>MADYKDDDDKSGRMLNNLTDCEDGDGGANPGDGNPKESSPFINSTDTEKGKEYDGKNMALFEEEMDTSPMVSSLLSGLANYTNLPQGSREHEEAENNEGGKKKPVQAPRMGTFMGVYLPCLQNIFGVILFLRLTWVVGIAGIMESFCMVFICCSCTMLTAISMSAIATNGVVPAGGSYYMISRSLGPEFGGAVGLCFYLGTTFAGAMYILGTIEILLAYLFPAMAIFKAEDASGEAAAMLNNMRVYGTCVLTCMATVVFVGVKYVNKFALVFLGCVILSILAIYAGVIKSAFDPPNFPICLLGNRTLSRHGFDVCAKLAWEGNETVTTRLWGLFCSSRFLNATCDEYFTRNNVTEIQGIPGAASGLIKENLWSSYLTKGVIVERSGMTSVGLADGTPIDMDHPYVFSDMTSYFTLLVGIYFPSVTGIMAGSNRSGDLRDAQKSIPTGTILAIATTSAVYISSVVLFGACIEGVVLRDKFGEAVNGNLVVGTLAWPSPWVIVIGSFFSTCGAGLQSLTGAPRLLQAISRDGIVPFLQVFGHGKANGEPTWALLLTACICEIGILIASLDEVAPILSMFFLMCYMFVNLACAVQTLLRTPNWRPRFRYYHWTLS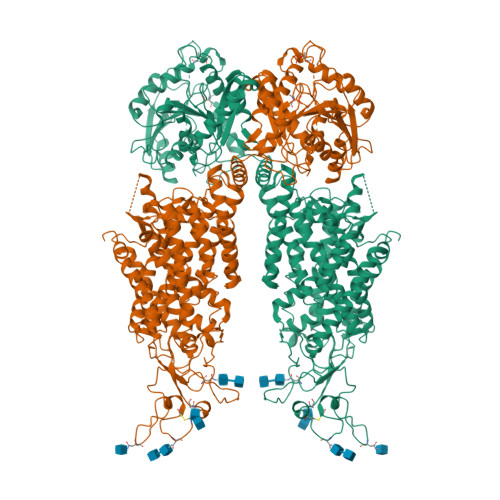FLGMSLCLALMFICSWYYALVAMLIAGLIYKYIEYRGAEKEWGDGIRGLSLSAARYALLRLEEGPPHTKNWRPQLLVLVRVDQDQNVVHPQLLSLTSQLKAGKGLTIVGSVLEGTFLENHPQAQRAEESIRRLMEAEKVKGFCQVVISSNLRDGVSHLIQSGGLGGLQHNTVLVGWPRNWRQKEDHQTWRNFIELVRETTAGHLALLVTKNVSMFPGNPERFSEGSIDVWWIVHDGGMLMLLPFLLRHHKVWRKCKMRIFTVAQMDDNSIQMKKDLTTFLYHLRITAEVEVVEMHESDISAYTYEKTLVMEQRSQILKQMHLTKNEREREIQSITDESRGSIRRKNPANTRLRLNVPEETAGDSEEKPEEEVQLIHDQSAPSCPSSSPSPGEEPEGEGETDPEKVHLTWTKDKSVAEKNKGPSPVSSEGIKDFFSMKPEWENLNQSNVRRMHTAVRLNEVIVKKSRDAKLVLLNMPGPPRNRNGDENYMEFLEVLTEHLDRVMLVRGGGREVITIYS[2x]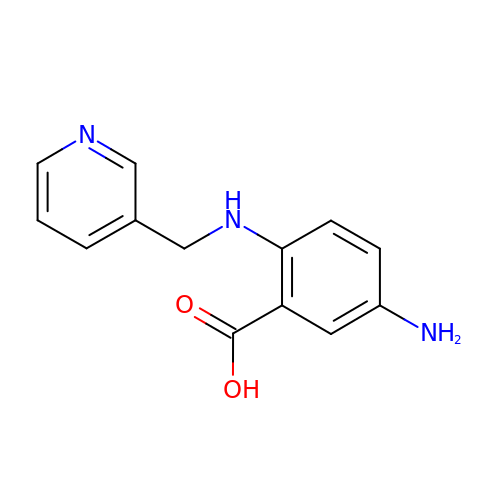5-azanyl-2-(pyridin-3-ylmethylamino)benzoic acid | C13 H13 N3 O2 | QEGXPJYAQLFLGN-UHFFFAOYSA-N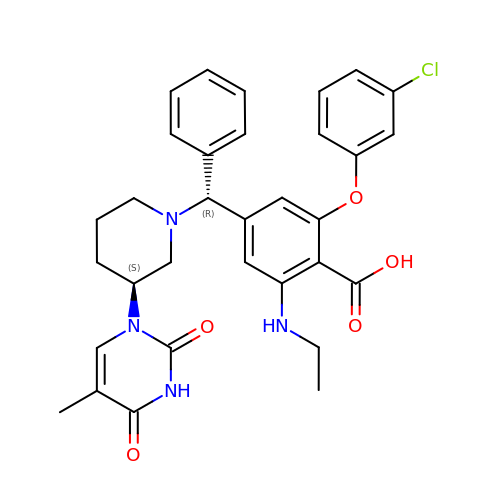2-(3-chlorophenoxy)-6-(ethylamino)-4-[(R)-[(3S)-3-(5-methyl-2,4-dioxo-3,4-dihydropyrimidin-1(2H)-yl)piperidin-1-yl](phenyl)methyl]benzoic acid | C32 H33 Cl N4 O5 | XESNVVRXJFEIMM-PWUYWRBVSA-N>[2x]GSHMSGRVGDLSPRQKEALAKFRENVQDVLPALPNPDDYFLLRWLRARSFDLQKSEAMLRKHVEFRKQKDIDNIISWQPPEVIQQYLSGGMCGYDLDGCPVWYDIIGPLDAKGLLFSASKQDLLRTKMRECELLLQECAHQTTKLGRKVETITIIYDCEGLGLKHLWKPAVEAYGEFLCMFEENYPETLKRLFVVKAPKLFPVAYNLIKPFLSEDTRKKIMVLGANWKEVLLK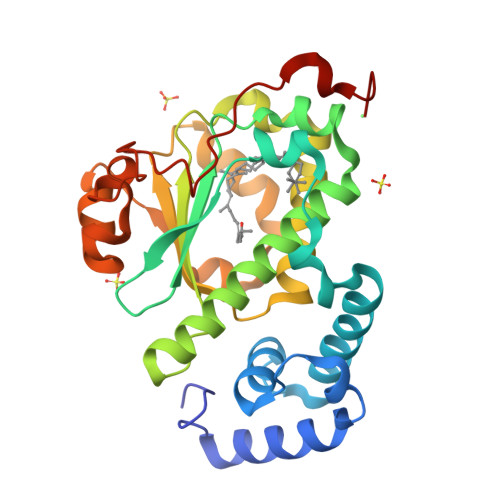HISPDQVPVEYGGTMTDPDGNPKCKSKINYGGDIPRKYYVRDQVK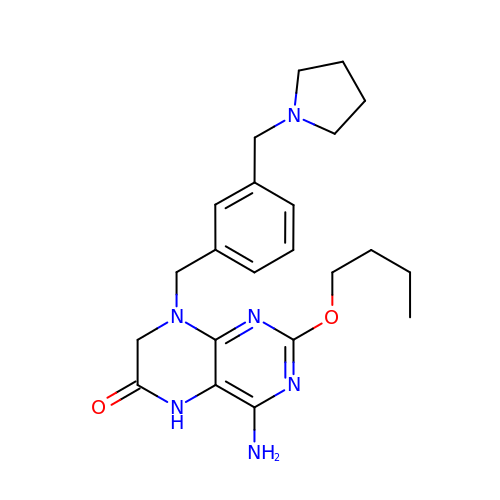4-azanyl-2-butoxy-8-[[3-(pyrrolidin-1-ylmethyl)phenyl]methyl]-5,7-dihydropteridin-6-one | C22 H30 N6 O2 | VFOKSTCIRGDTBR-UHFFFAOYSA-N>[2x]QNVSLQPPPQQLIVQNKTIDLPAVYQLNGGEEANPHAVKVLKELLSGKQSSKKGMLISIGEKGDKSVRKYSRQIPDHKEGYYLSVNEKE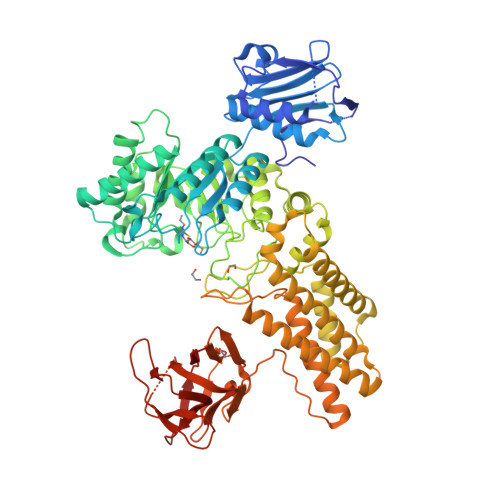IVLAGNDERGTYYALQTFAQLLKDGKLPEVEIKDYPSVRYRGVVEGFYGTPWSHQARLSQLKFYGKNKMNTYIYGPKDDPYHSAPNWRLPYPDKEAAQLQELVAVANENEVDFVWAIHPGQDIKWNKEDRDLLLAKFEKMYQLGVRSFAVFFDDISGEGTNPQKQAELLNYIDEKFAQVKPDINQLVMCPTEYNKSWSNPNGNYLTTLGDKLNPSIQIMWTGDRVISDITRDGISWINERIKRPAYIWWNFPVSDYVRDHLLLGPVYGNDTTIAKEMSGFVTNPMEHAESSKIAIYSVASYAWNPAKYDTWQTWKDAIRTILPSAAEELECFAMHNSDLGPNGHGYRREESMDIQPAAERFLKAFKEGKNYDKADFETLQYTFERMKESADILLMNTENKPLIVEITPWVHQFKLTAEMGEEVLKMVEGRNESYFLRKYNHVKALQQQMFYIDQTSNQNPYQPGVKTATRVIKPLIDRTFATVVKFFNQKFNAHLDATTDYMPHKMISNVEQIKNLPLQVKANRVLISPANEVVKWAAGNSVEIELDAIYPGENIQINFGKDAPCTWGRLEISTDGKEWKTVDLKQKESRLSAGLQKAPVKFVRFTNVSDEEQQVYLRQFVLTIEKK>[2x]IIGGHEVTPHSRPYMASVRFGGQHHCGGFLLRARWVVSAAHCFSHRDLRTGLVVLGAHVLSTAEPTQQVFGIDALTTHPDYHPMTHANDICLLR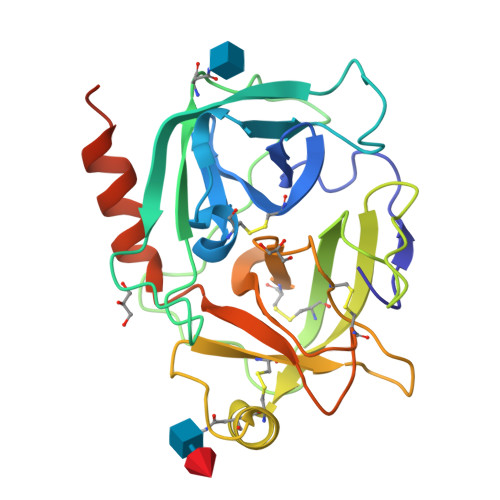LNGSAVLGPAVGLLRLPGRRARPPTAGTRCRVAGWGFVSDFEELPPGLMEAKVRVLDPDVCNSSWKGHLTLTMLCTRSGDSHRRGFCSADSGGPLVCRNRAHGLVSFSGLWCGDPKTPDVYTQVSAFVAWIWDVVRRSSPQPGPLPGTTRPPGEAA>[2x]GPLGSMGKKSRVKTQKSGTGATATVSPKEILNLTSELLQKCSSPAPGPGKEWEEYVQIRTLVEKIRKKQKGLSVTFDGKREDYFPDLMKWASENGASVEGFEMVNFKEEGFGLRATRDIKAEELFLWVPRKLLMTVESAKNSVLGPLYSQDRILQAMGNIALAFHLLCERASPNSFWQPYI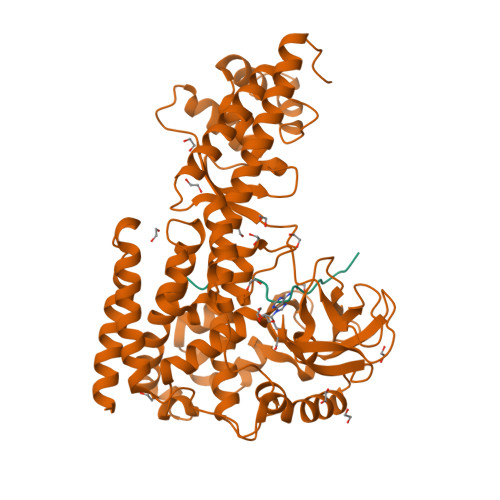QTLPSEYDTPLYFEEDEVRYLQSTQAIHDVFSQYKNTARQYAYFYKVIQTHPHANKLPLKDSFTYEDYRWAVSSVMTRQNQIPTEDGSRVTLALIPLWDMCNHTNGLITTGYNLEDDRCECVALQDFRAGEQIYIFYGTRSNAEFVIHSGFFFDNNSHDRVKIKLGVSKSDRLYAMKAEVLARAGIPTSSVFALHFTEPPISAQLLAFLRVFCMTEEELKEHLLGDSAIDRIFTLGNSEFPVSWDNEVKLWTFLEDRASLLLKTYKTTIEEDKSVLKNHDLSVRAKMAIKLRLGEKEILEKAVKSAAVNREYYRQQMEEKAPLPKYEESNLGLLESSVGDSRLPLVLRNLEEEAGVQDALNIREAISKAKATENGLVNGENSIPNGTRSENESLNQESKRAVEDAKGSSSDSTAGVKE;>TLKYPIEHGIVTNWD[2x]>[2x]WQENKSWNAHFTEHKSQGVVVLWNENKQQGFTNNLKRANQAFLPASTFKIPNSLIALDLG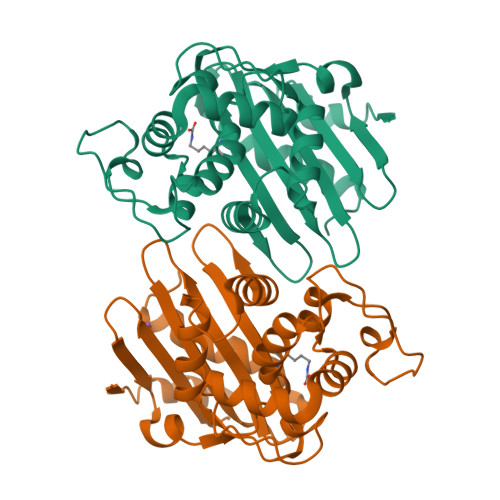VVKDEHQVFKWDGQTRDIATWNRDHNLITAMKYSVVPVYQEFARQIGEARMSKMLHAFDYGNEDISGNVDSFWLDGGIRISATEQISFLRKLYHNKLHVSERSQRIVKQAMLTEANGDYIIRAKTGYDTKIGWWVGWVELDDNVWFFAMNMDMPTSDGLGLRQAITKEVLKQEKIIP> ANPPGGDPDPGCQTDCNYQCGPDPTDAYLEAASGPYTVSTIRVSSLVPGFGGGTIHYPTNACGGKMAGIVVIPGYLSRESSIKWWGPRLASHGFVVMTIDTNTIYDQPSQRRDQIEAALQYLVNQSNSPSSPISG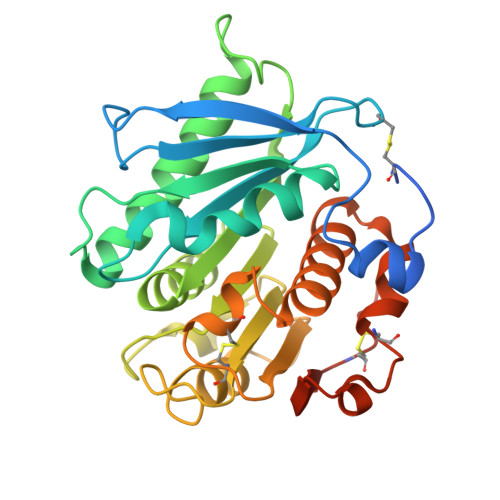MVDSSRLAAVGWSMGGGATLQLAADGGIKAAIALAPWNSSINDFNRIQVPTLIFACQLDAIAPVALHASPFYNRIPNTTPKAFFEMTGGDHWCANGGNIYSALLGKYGVSWMKLHLDQDTRYAPFLCGPNHAAQPLISEYRGNCPYENLYFQGHHHHHH>MVVRRTVLKAIAGTSVATVFAGKLTGLSAVAADAAPLRVRRNLHGMKMDDPDLSAYREFVGIMKGKDQTQALSWLGFANQHGTLNGGYKYCPHGDWYFLPWHRGFVLMYERAVAALTGYKTFAMPYWNWTEDRLLPEAFTAKTYNGKTNPLYVPNRNELTGPYALTDAIVGQKEVMDKIYAETNFEVFGTSRSVDRSVRPPLVQNSLDPKWVPMGGGNQGILERTPHNTVHNNIGAFMPTAASPRDPVFMMHHGNIDRVWATWNALGRKNSTDPLWLGMKFPNNYIDPQGRYYTQGVSDLLSTEALGYRYDVMPRADNKVVNNARAEHLLALFKTGDSVKLADHIRLRSVLKGEHPVATAVEPLNSAVQFEAGTVTGALGADVGTGSTTEVVALIKNIRIPYNVISIRVFVNLPNANLDVPETDPHFVTSLSFLTHAAG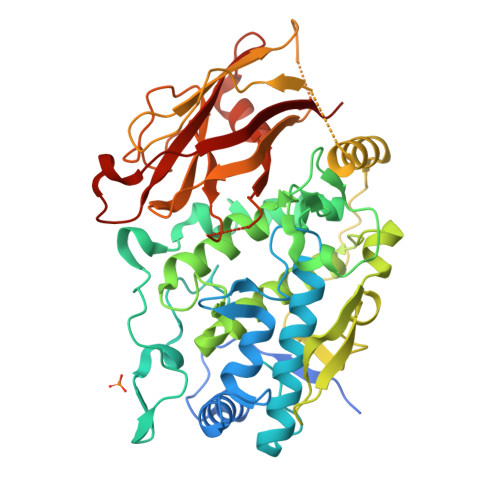HDHHALPSTMVNLTDTLKALNIRDDNFSINLVAVPQPGVAVESSGGVTPESIEVAVIA[3x]>CCCGCGGG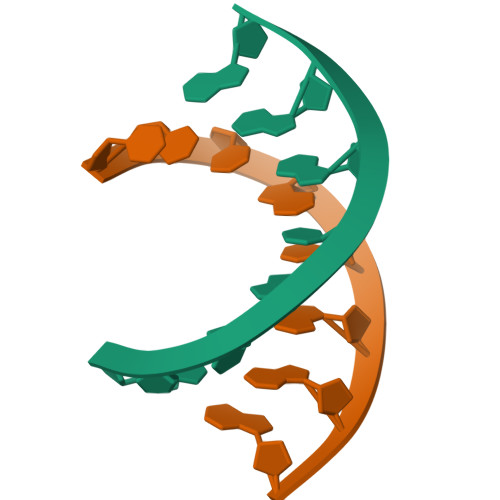[2x]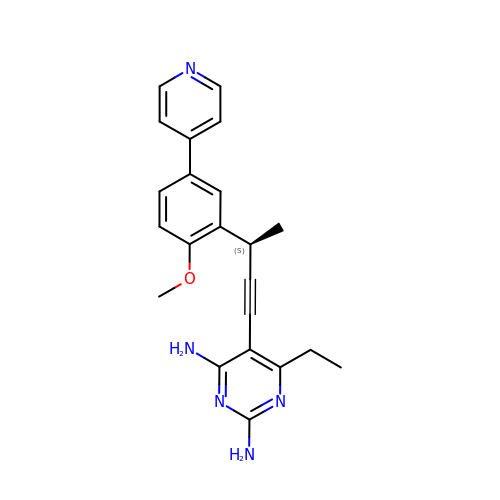6-ethyl-5-{(3S)-3-[2-methoxy-5-(pyridin-4-yl)phenyl]but-1-yn-1-yl}pyrimidine-2,4-diamine | C22 H23 N5 O | PPKWGSTVAQFAGZ-AWEZNQCLSA-N> MPKTISVRVTTMDAELEFAIQPNTTGKQLFDQVVKTIGLREVWFFGLQYQDTKGFSTWLKLNKKVTAQDVRKESPLLFKFRAKFYPEDVSEELIQDITQRLFFLQVKEGILNDDIYCPPETAVLLASYAVQSKYGDFNKEVHKSGYLAGDKLLPQRVLEQHKLNKDQWEERIQVWHEEHRGMLREDAVLEYLKIAQDLEMYGVNYFSIKNKKGSELWLGVDALGLNIYEQNDRLTPKIGFPWSEIRNISFNDKKFVIKPIDKKAPDFV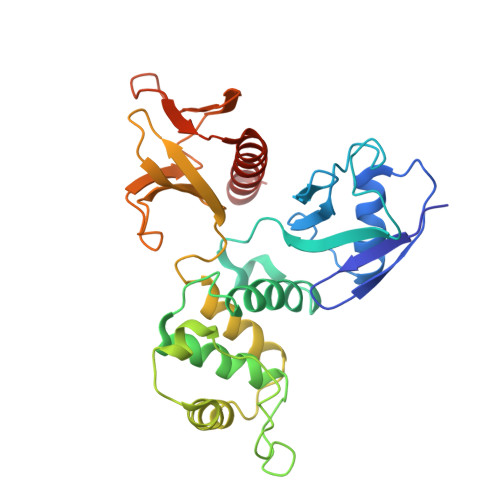FYAPRLRINKRILALCMGNHELYMRRRKP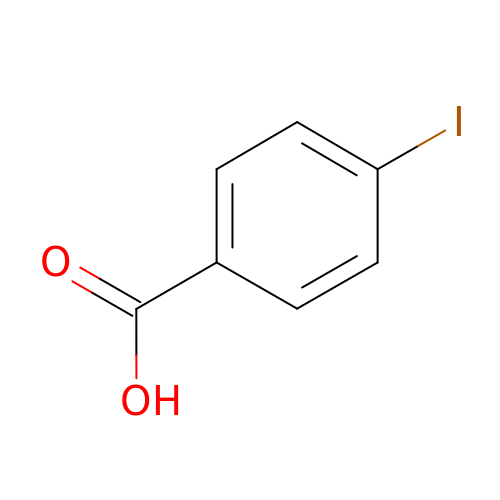4-iodobenzoic acid | C7 H5 I O2 | GHICCUXQJBDNRN-UHFFFAOYSA-N The defense-associated sirtuin 2 (DSR2) effector, a SIR2 domain-containing protein, protects bacteria from phage infection by depleting NAD+, while an anti-DSR2 protein (DSR anti-defense 1, DSAD1) is employed by some phages to evade this host defense. The NADase activity of DSR2 is unleashed by recognizing the phage tail tube protein (TTP). DSR2 is arranged as a dimer of dimers, which is facilitated by the tetramerization of SIR2 domains. DSR2 has a two-domain architecture, with the CTD responsible for sensing the infection signal and SIR2 acting to prevent phage propagation.

We therefore reconstituted the DSR2-DSAD1 binary complex and determined the cryo-EM structures at resolutions of 3.4–3.6 Å. DSAD1 is trapped by the tip of the CTD fishhook. Particularly, sheet-2 of DSAD1 packs above the H3 subdomain. The H4 subdomain, along with the H3 subdomain from the adjacent molecule, brackets the β-hairpin of DSAD1. Notably, Tyr16 of DSAD1 stacks against Tyr574 and Phe576 from the adjacent H3 subdomain. The interaction between DSR2 and DSAD1 was significantly compromised when mutating Tyr574 and Phe576 to glycine, indicating that the formation of DSR2 dimer appears to be important for DSAD1 binding. While the overall structure of the DSR2 molecule in the absence of DSAD1 is similar to that of the DSAD1-bound DSR2 molecule, subtle structural discrepancies are discerned within the H4 subdomain. The H4 subdomain moves outward by ~10 Å to accommodate DSAD1. The H4 subdomain seems to be critical for DSAD1 binding, as supported by the fact that the H4 subdomain and DSAD1 constitute the largest interface between DSR2 and DSAD1. Furthermore, DSAD1 was compromised in binding to DSR2 protein upon the removal of the H4 subdomain.

>[4x]MVKVDLESKRYGEKLKEVFLMLDNNVVECIKEITESSRNGKLVFFVGAGVSTLSDYPQWWRLVDKYHEELYGSPKKGNYSSDEYLRIPQIFYNVKGEMAFDGILKDFFQVDKPTNPIHDKILAMNPAHVITTNYDNLIDTACWKRGKYFSVISAEEDVANATSSRYLLKVHGDFRKGFKGENVVLKEDDYLNYDQNYPLISNLMKTIIATHTIVFIGYGLGDYNINMLLNWVRKLQKDSFHKPFFIRTDPSPIENETLIYYENKGLRIIDAASLIDSNEYDYLERYSAVMDLLIESQENKFITKDDEVIDYIYGKISPLFALQYIRKIDLKHVFEYDYHFEVNGTVVRHKNKGFGYMERFFELKESCDERSKLSKKQYERFNALFNFFEKNGVICMAKDAGTLNTSIEINSLAYHGKYDVMKKFIEEQSVSIEDDYKKAFFLACLGRWEESYDLYSNIILNSIDESNGCVYYLSQINRYRIYQSITQAVTQFNGLGLLTFGRHYKPFTDEFLARIEREMTNFNIDDLFNGMPFEFQKKYKILEFLSDNQFLYDDTVKLFELTNKVRSEMSEGSYSFGMSSDIVVLLRLYDNLRFLYENCLWSVSFHEFHQYIRNSMSLLIEKAEYERTRDIDELGFSFFGKKSGFFMEYYDFVNISRHFKIDDIKNLERSCSIDKIRFGEQEKIEEYLVGIAEEITKQFSANGMNVVFYTQFISEAKAALYFAKYVKLSEEGLGKIVKALLFYFPERDLDIGKRYVWLERLTKCNELPKSIISIIDDFLVLQAEKHIDQNYSEVSSNGLYSRDYGALIKHFEKNFISKRLSEITLCLTQDKQKQIDFLFKLLPLLSTNAKSHLLSFKSVENINDLMNGIRIGLIDEFTPEHEELIIEYLETRKVNYIVEKEKGIQTFSSNDYMSTFGIWYFLEEINNSKMEEFIGMDDQYDFFVDPENFDYKKFIPSWLKNYNDKLLGKIAGNKHMKHHVIEVLKERVKNSNDKRYLEILMNYFI;> MIEIFKDTGATHDLVYHSKINTFVWDVEFDIVLSDSKELNKCYFVKCFNPYRINGKCDFAVSSIDIFSEGKRLLIENEFNFKITKAVHVATSKDVTEIVLHLSERISSPFPIVKEVVYLD>[2x]GPLGSSMEDHDDHLRRKFMEFPYVSPTRKQLMVDLMSTVENRLQSQLLPCNLPPDVRNFNNPNGSAEASLHIRSGDKSSPIDFVIGSWIHCKIPTGVSLNITSISGFLNSSTKAPNFVVELIQSSSKSLVLILDLPHRKDLVLNPDYLKEYYQDTALDSHRQSLLKLPEVNPYVSPSLFVRSAFSPTASMLKID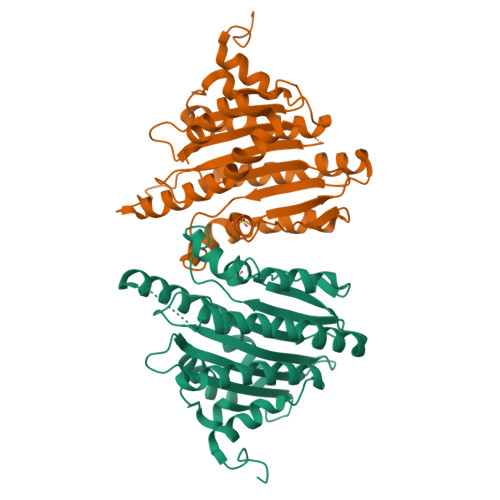AEEEDKLEEILRDHVSPAAKEVLEVWLERCVKEEEEKIVVGEEERMELERRDKSFRRKSIEDDLDLQFPRMFGEEVSSRVVHAIKEAFGVL> PISPIETVPVKLKPGMDGPKVKQWPLTEEKIKALVEICTEMEKEGKISKIGPENPYNTPVFAIKKKDSTKWRKLVDFRELNKRTQDFWEVQLGIPHPAGLK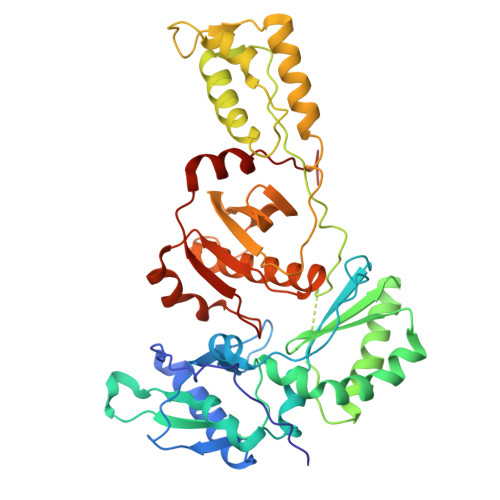KKKSVTVLDVGDAYFSVPLDEDFRKYTAFTIPSINNETPGIRYQYNVLPQGWKGSPAIFQSSMTKILEPFKKQNPDIVIYQYMDDLYVGSDLEIGQHRTKIEELRQHLLRWGLTTPDKKHQKEPPFLWMGYELHPDKWTVQPIVLPEKDSWTVNDIQKLVGKLNWASQIYPGIKVRQLCKLLRGTKALTEVIPLTEEAELELAENREILKEPVHGVYYDPSKDLIAEIQKQGQGQWTYQIYQEPFKNLKTGKYARMRGAHTNDVKQLTEAVQKITTESIVIWGKTPKFKLPIQKETWETWWTEYWQATWIPEWEFVNTPPLVKLWYNLEKEPIVGAETF Here we present a series of TIGR03971 SDR crystal structures from several mycobacterial species which contain an insertion in the primary sequence at the NAD cofactor binding site. These crystal structures demonstrate that the inserted protein residues almost completely cover the NAD cofactor, only leaving part of the nicotinamide ring exposed to solvent. NMR experiments did not show exchange of the NAD cofactor, whereas binding was demonstrated for a number of small molecules which could be potential substrates, products, inhibitors, or artificial redox partners. Experimental results are consistent with the notion that the SDR family enzymes linked by comparative genomics studies to mycofactocin do indeed keep their NAD tightly bound beneath a protein structure that may interact with a specialized adaptor machinery for redox exchange.

With the exception of the M. thermoresistibile target which did not contain NAD, all other mycobacterial SDR target crystal structures contained NAD, which appears to have co-purified with the protein after expression in E. coli. For each of these crystal structures, the adenosine mononucleotide portion of the cofactor binding site is enveloped by the inserted residues and only a portion of the nicotinamide ring appears open to solvent (see representative examples in Fig. 2A and B). In addition to the insertion loop which covers the adenosine portion of the cofactor, a second loop which typically contains two α-helices covers much of nicotinamide mononucleotide portion of the cofactor. In contrast, this loop is ordered in each of the mycobacterial SDR crystal structures presented here. The combination of the insertion loop which covers the adenosine portion of the cofactor and the ordering of the second loop which covers the nicotinamide mononucleotide portion of the cofactor results in a significant decrease in the solvent accessible surface area of the cofactor in the mycobacterial SDRs, relative to other NAD- and NADP-dependent dehydrogenases. Only a small portion of the nicotinamide ring appears available to solvent in each of these cases, indicating that the NAD cofactor is tightly bound and potentially non-exchangeable. The structures presented here have a cofactor solvent accessible surface area of approximately 18 Å2, whereas other NAD- or NADP-bound dehydrogenases have a cofactor solvent accessible surface area of 82–89 Å2. Given the encapsulation of the NAD cofactor by the two loops in mycobacterial SDRs, a large conformational change would be required to release the NADH cofactor after a redox reaction had occurred. Alternatively, these structural elements may not allow for exchange of bound NAD/NADH with free NAD/NADH.

>[8x]GPGSMADFEGKTALITGGARGMGRSHAVALAEAGADIAICDRCENSDVVGYPLATADDLAETVALVEKTGRRCISAKVDVKDRAALESFVAEAEDTLGGIDIAITNAGISTIALLPEVESAQWDEVIGTNLTGTFNTIAAVAPGMIKRNYGRIVTVSSMLGHSANFAQASYVSSKWGVIGLTKCAAHDLVGYGITVNAVAPGNIETPMTHNDFVFGTMRPDLEKPTLKDVESVFASLHLQYAPFLKPEEVTRAVLFLVDEASSHITGTVLPIDAGATARMI>[2x]GQKKSIYVAYTGGTIGMQRSDNGYIPVSGHLQRQLALMPEFHDPEMPDFTIHEYAPLIDSSDMTPEDWQHIANDIQQNYDLYDGFVILHGTDTMAFT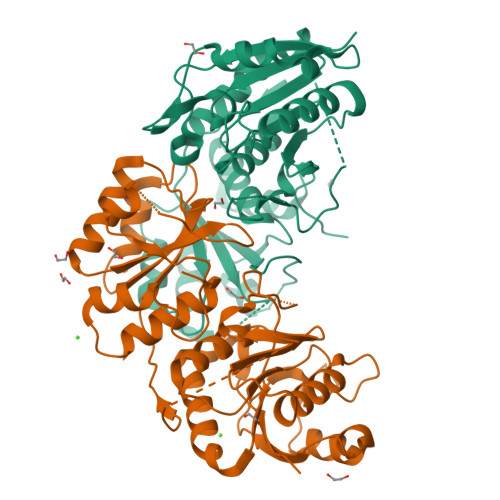ASALSFMLENLAKPVIITGSQIPLAEDASDGQTNLLNALYLAANHPVNEVSLFFNNQLFRGNRTTKAHADGFDAFASPNLSVLLEAGIHIRRQSSVVSPTSNGPLIVHRITPQPIGVVTIYPGISGAVVRNFLLQPVKALILRSYGVGNAPQKAELLDELKNASDRGIVVVNLTQSISGSVNMGGYATGNALAQAGVISGFDMTVEAALTKLHYLLSQSLSPNEIRQLMQQNLRGELTDTQ>QTSCDQWATFTGNGYTVSNNLWGASAGSGFGCVTAVSLSGGASWHADWQWSGGQNNVKSYQNSQIAIPQKRTVNSISSMPTTASWSYSGSNIRANVAYDLFTAANPNHVTYSGDYELMIWLGKYGDIGPIGSSQGTVNVGGQSWTLYYGYNGAMQVYSFVAQTNTTNYS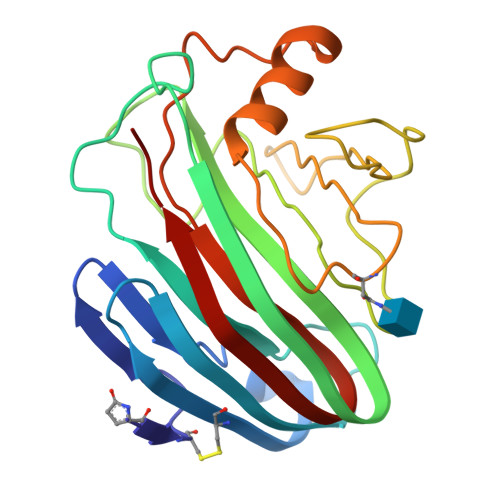GDVKNFFNYLRDNKGYNAAGQYVLSYQFGTECFTGSGTLNVASWTASIN[2x]>[2x]EEVRQFRRLFAQLAGDDMEVSATELMNILNKVVTRHPDLKTDGFGIDT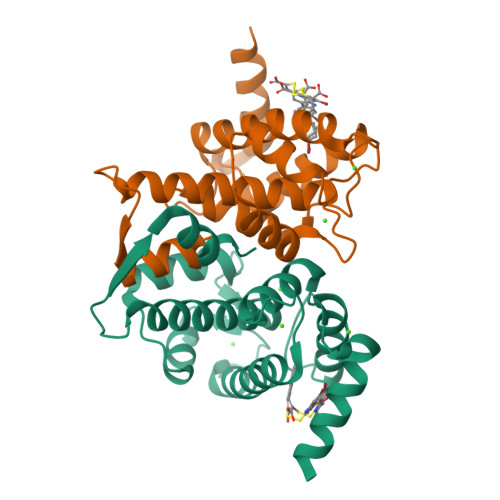CRSMVAVMDSDTTGKLGFEEFKYLWNNIKRWQAIYKQFDTDRSGTICSSELPGAFEAAGFHLNEHLYNMIIRRYSDESGNMDFDNFISCLVRLDAMFRAFKSLDKDGTGQIQVNIQEWLQLTMYS> TTIVSVRRNGHVVIAGDGQATLGNTVMKGNVKKVRRLYNDKVIAGFAGGTADAFTLFELFERKLEMHQGHLVKAAVELAKDWRTDRMLRKLEALLAVADETASLIITGNGDVVQPENDLIAIGSGGPYAQAAARALLENTELSAREIAEKALDIAGDICIYT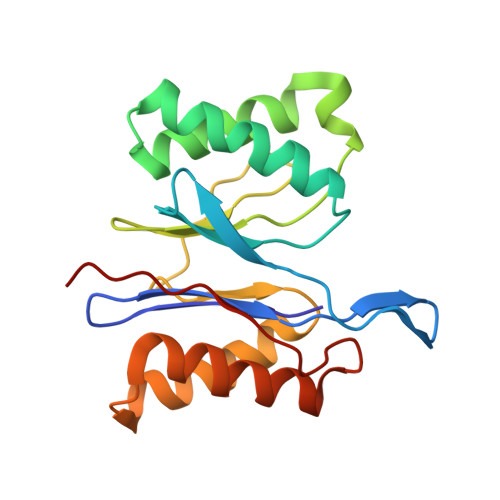NHFHTIEELSYKA> MERTELLKPRTLADLIRILHELFAGDEVNVEEVQAVLEAYESNPAEWALYAKFDQYRYTR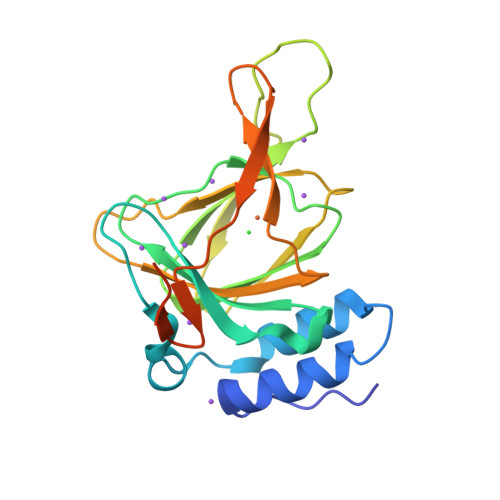NLVDQGNGKFNLMILCWGEGHGSSIHDHTDSHCFLKLLQGNLKETLFDWPDKKSNEMIKKSERTLRENQCAYINDSIGLHRVENVSHTEPAVSLHLFSPPFDTCHAFDQRTGHKNKVTMTFHSKFGIRTPFTTSGSLENNSAWSHPQFEK> HMAELRRQGVAPTVVTYNALIDGLCKAGKLDEALKLFEEMVEKGIKPDEFTFSSVLKACARLGALELGKQIHGYVIKS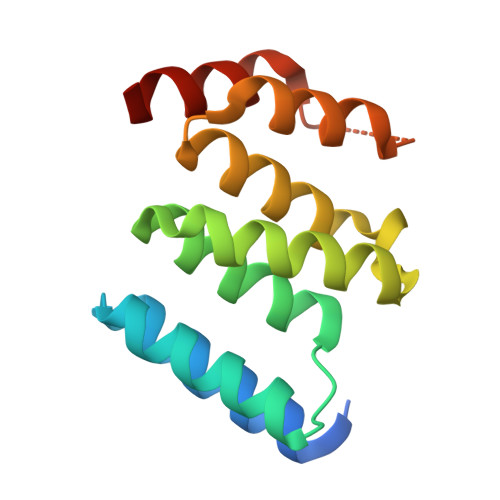GFESNVVVYNALIDMYSKCGLLEEARKVFDEMPEKDELTYRRVVESYCRAKRFE>MDLAPQMLRELQE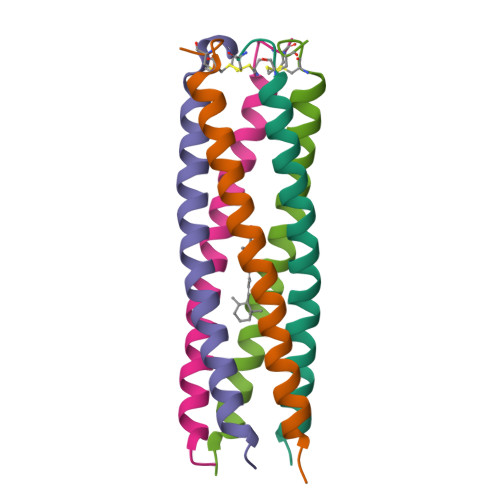TNAALQDVRELLRQQVKEITFLKNTVMECDACG[5x]>[6x]MAGNKPFNKQQAEPRERDPQVAGLKVPPHSIEAEQSVLGGLMLDNERWDDVAERVVADDFYTRPHRHIFTEMARLQESGSPIDLITLAESLERQGQLDSVGGFAYLAELSKNTPSAANISAYADIVRERAVVREMISVANEIAEAGFDPQGRTSEDLLDLAESRVFKIAESRANKDEGPKNIADVLDATVARIEQLFQ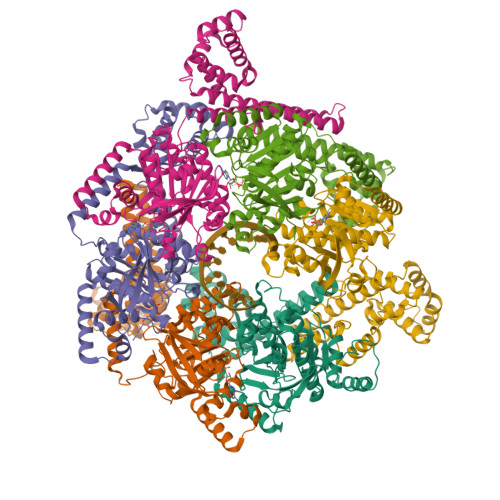QPHDGVTGVNTGYDDLNKKTAGLQPSDLIIVAARPSMGKTTFAMNLVENAAMLQDKPVLIFSLEMPSEQIMMRSLASLSRVDQTKIRTGQLDDEDWARISGTMGILLEKRNIYIDDSSGLTPTEVRSRARRIAREHGGIGLIMIDYLQLMRVPALSDNRTLEIAEISRSLKALAKELNVPVVALSQLNRSLEQRADKRPVNSDLRESGSIEQDADLIMFIYRDEVYHENSDLKGIAEIIIGKQRNGPIGTVRLTFNGQWSRFDNYAGPQYDDE2,3-dichloro-N-{2-[formyl(hydroxy)amino]ethyl}benzamide | C10 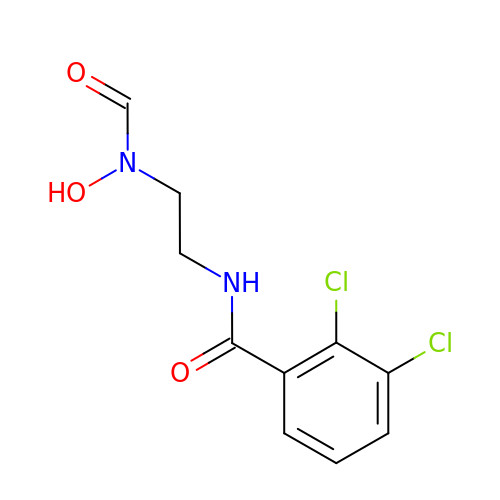H10 Cl2 N2 O3 | QOBOQKAHMKWYEE-UHFFFAOYSA-N>GGKKKVCYYYDGDIGNYYYGQGHPMKPHRIRMTHNLLL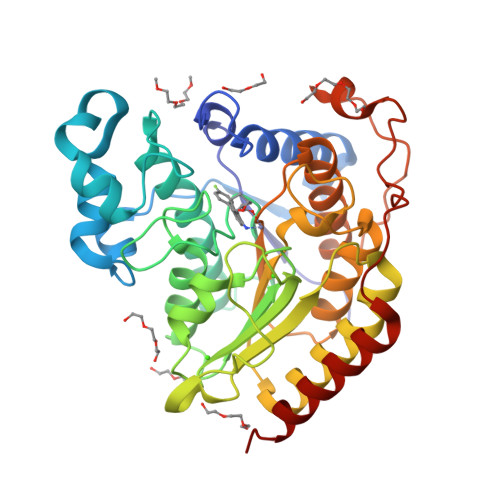NYGLYRKMEIYRPHKATAEEMTKYHSDEYIKFLRSIRPDNMSEYSKQMQRFNVGEDCPVFDGLFEFCQLSTGGSVAGAVKLNRQQTDMAVNWAGGLHHAKKSEASGFCYVNDIVLAILELLKYHQRVLYIDIDIHHGDGVEEAFYTTDRVMTVSFHKYGEYFPGTGDLRDIGAGKGKYYAVNFPMRDGIDDESYGQIFKPIISKVMEMYQPSAVVLQCGADSLSGDRLGCFNLTVKGHAKCVEVVKTFNLPLLMLGGGGYTIRNVARCWTYETAVALDCEIPNELPYNDYFEYFGPDFKLHISPSNMTNQNTPEYMEKIKQRLFENLRMLP[3x]3-[[(2~{R},3~{S},4~{R},5~{R})-5-(2-azanyl-7-methyl-6-oxidanylidene-1~{H}-purin-7-ium-9-yl)-3,4-bis(oxidanyl)oxolan-2-yl]methylamino]-4-oxidanyl-cyclobut-3-ene-1,2-dione 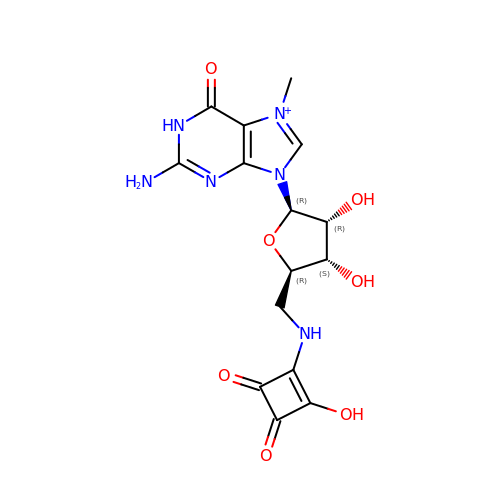| C15 H17 N6 O7 | WRZJZJPEHQGNLE-CZCBHZRKSA-O2,3-DI-PHYTANYL-GLYCEROL | C43 H88 O3 | 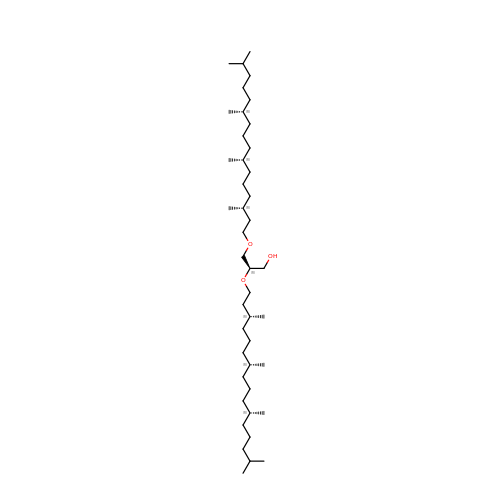ISDBCJSGCHUHFI-UMZPFTBHSA-N>GAGTVASVAGTATASGIASGTVNLVGGGQVKNIAIAAGDSAKAIAEKMDGAIPNLSARARTVFTADVSGVTGGSLNFDVTVGSNTVSLAGVTSTQDLADQLNSNSSKLGITASINDKGVLTITSATGENVKFGAQTGTATAGQVAVKVQGSDGKFEAAAKNVVAAGTAATTTIVTGYVQLNSPTAYSVSGTGTQASQVFGNASAAQKSSVASVDISTA[2x]

The flagellar filament, a tubular structure composed of thousands of copies of the protein flagellin (FliC in many bacteria), exhibits helical symmetry in its straight non-motile forms and is supercoiled with a three-dimensional waveform in motile bacteria. Flagellar filaments can be neatly divided structurally into the two highly conserved inner domains, D0 and D1, which form the inner core of the filament, and a diverse number of outer domains, which decorate the inner core. Here we show that in the Pseudomonas aeruginosa PAO1 strain, a bacterium that forms a ridged filament with a dimerization of its flagellin outer domains, motility is categorically dependent on these flagellin outer domains. Moreover, a comprehensive network of intermolecular interactions connecting the inner domains to the outer domains, the outer domains to one another, and the outer domains back to the inner domain filament core, is required for motility.

Although the cryo-EM structure of the PAO1 filament achieved near-atomic resolution for the inner core of the filament, the resolution of the outer domains was substantially lower, prohibiting even the tracing of the main chain of the D2 and D3 domains. Thus, we expressed and purified the fragment of FliC between residues 178–395 that forms the D2 and D3 domains and crystallized both the native protein and its selenomethionine derivative in the P2 space group with 2 molecules in the asymmetric unit. Employing multi-wavelength anomalous dispersion (MAD) phasing methods, we arrived at a 1.47 Å resolution structure revealing the D2 and D3 domains as a contiguous barrel-like structure composed predominantly of β-strands, with D3 positioned directly above D2 along the filament axis towards the distal end of the filament. While D3 in S. Typhimurium is inserted into D2 and they form two separated domains, a different topology of the secondary structural elements in PAO1 FliC results in the D2 and D3 domains folding into a single bilobal structure with two distinct surfaces, the concave surface facing the filament core, and the convex surface exposed to the outside. Starting from the N-terminus, the first β-strand is incorporated into the D3 moiety, before the backbone turns downward, forming one half of D2. The sequence between 243 and 353 is entirely a part of D3, after which the polypeptide chain returns to complete the fold of D2. On the concave side of the D2/D3 domain, residues between 233 and 242 belong to the β4-strand that occupies central position spanning both D2 and D3 and together with strands 7, 8, 10 and 11 of D3 and strand 13 of D2 they form an antiparallel β-sheet. The consequence of this organization is the tight packing of D2 and D3 which are oriented along the filament, instead of projecting away from it as in the S. Typhimurium. Compared to the previously determined structure of the type A PAK FliC, our type B PAO1 FliC outer domains are oriented similarly relative to the inner core.>[4x]MAATSSTSSQSFDIELDIIGQQPPLLSIYTQISLVYPVSDPSQYPTIVSTLEEGLKRLSQTFPWVAGQVKTEGISEGNTGTSKIIPYEETPRLVVKDLRDDSSAPTIEGLRKAGFPLEMFDENVVAPRKTLAIGPGNGPNDP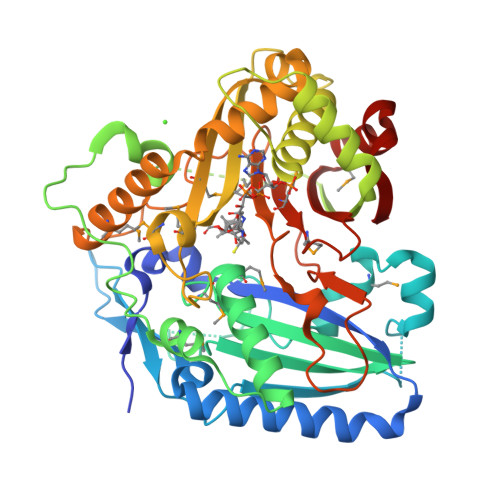KPVLLLQLNFIKGGLILTVNGQHGAMDMTGQDAIIRLLSKACRNESFTEEEISAMNLDRKTVVPLLENYKVGPELDHQIAKPAPAGDAPPAPAKATWAFFSFTPKALSELKDAATKTLDASSKFVSTDDALSAFIWQSTSRVRLARLDASTPTEFCRAVDMRGPMGVSSTYPGLLQNMTYHDSTVAEIANEPLGATASRLRSELNSDRLRRRTQALATYMHGLPDKSSVSLTADANPSSSIMLSSWAKVGCWEYDFGFGLGKPESVRRPRFEPFESLMYFMPKKPDGEFTASISLRDEDMERLKADEEWTKYAKYIG> MGSGQEHALENYWPVMGVEFSEDMLDFPALFGREAPVTLEIGFGMGASLVAMAKDRPEQDFLGIEVHSPGVGACLASAHEEGLSNLRVMCHDAVEVLHKMIPDNSLRMVQLFF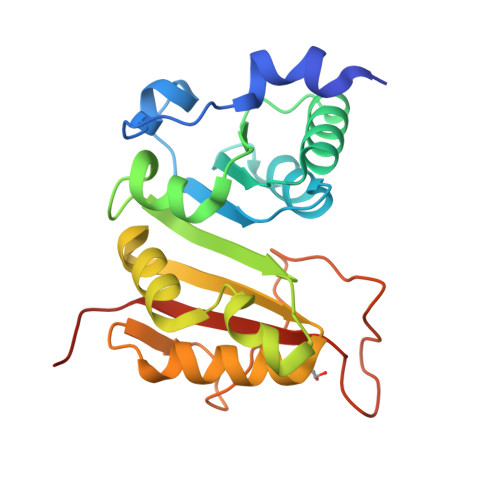PDPWHKARHNKRRIVQVPFAELVKSKLQLGGVFHMATDWEPYAEHMLEVMSSIDGYKNLSESNDYVPRPASRPVTKFEQRGHRLGHGVWDLMFERVKLEHHHHHH>HMQKVEVFRIPTASPDDISGLATLIDSGKINPAEIVAILGKTEGNGCVNDFTRGFATQSLAMYLAEKLGISREEVVKKVAFIMSGGTEGVMTPHITVFVRKDVAAPAAPGKRLAVGVAFTRDFLPEELGRMEQVNEVARAVKEAMKDAQIDDPRDVHFVQIKCPLLTAERIEDAKRRGKDVVVNDTYKSMAYSRGASALGVALALGEISADKISNEAICHDWNLYSSVASTSAGVELLNDEIIVVGNSTNSASDLVIGHSVMKDAIDADAVRAALKDAG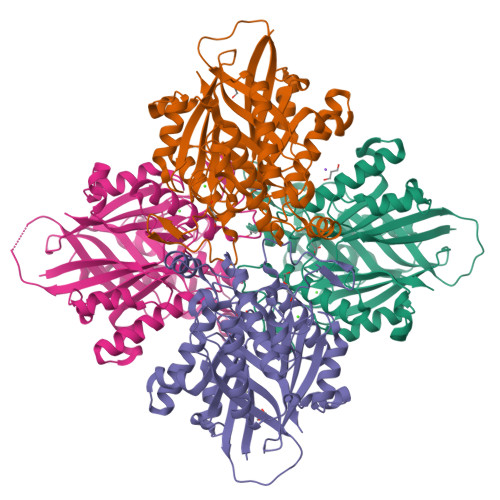IRSDDEMDRIVNVLAKAEAASSGTVRGRRNTMLDDSDINHTRSARAVVNAVIASVVGDPMVYVSGGAEHQGPDGGGPIAVIARV[4x]Phenolamides, also known as phenylamides or hydroxycinnamic acid amides, are ubiquitous secondary metabolites in plants. All these phenolamide synthesis enzymes belong to the acyl-coenzyme A (CoA)-dependent BAHD acyltransferases family, which was named according to the first letter of each of its first four biochemically characterized enzymes: Benzylalcohol O-acetyltransferase, Anthocyanin O-HCT, HCT of anthranilate, and Deacetylvindoline 4-O-acetyltransferase. It has been established that BAHD acyltransferases catalyze the transfer of acyl groups from acyl-donors (Acyl-CoA) to various acyl-acceptors. In this study, we first performed structural analyses on two representative BAHD family enzymes, the Arabidopsis mono-/di-acyltransferase-SDT (AtSDT) and poly acyltransferase-SHT (AtSHT), then explored the acceptor-molecule specificity and potential molecular mechanisms of multisite acylation by structure-based mutagenesis approaches, and, finally, successfully predicted and varified the acyl acceptor substrates of two uncharacterized BAHD family transferases in Arabidopsis using our prediction methods on the basis of a sequence similarity network (SSN) and of structure modeling.

In contrast to the mono- or di- substituted phenolamides, which seem to be widely distributed in different organs, the poly-substituted phenolamides, tri-substituted spermidine, and tetra-substituted spermidine were found to be restricted to the flower pollen coat. Spermidine/spermine hydroxycinnamoyl transferases (SHT), accounting for the synthesis of tri- or tetra- substituted spermidine/spermidine, have been identified and studied in Arabidopsis thaliana (AtSHT), Malus domestica (MdSHT), and Cichorium intybus (CiSHT; Grienenberger et al., 2009; Elejalde-Palmett et al., 2015; Delporte et al., 2018). In addition, the multisite acylation mechanisms of BAHD-family acyltransferases also remain poorly understood until now.

> MAPITFRKSYTIVPAEPTWSGRFPLAEWDQVGTITHIPTLYFYDKPSESFQGNVVEILKTSLSRVLVHFYPMAGRLRWLPRGRFELNCNAEGVEFIEAESEGKLSDFKDFSPTPEFENLMPQVNYKNPIETIPLFLAQVTKFKCGGISLSVNVSHAIVDGQSALHLISEWGRLARGEPLETVPFLDRKILWAGEPLPPFVSPPKFDHKEFDQPPFLIGETDNVEERKKKTIVVMLPLSTSQLQKLRSKANGSKHSDPAKGFTRYETVTGHVWRCACKARGHSPEQPTALGICIDTRSRMEPPLPRGYFGNATLDVVAASTSGELISNELGFAASLISKAIKNVTNEYVMIGIEYLKNQKDLKKFQDLHALGSTEGPFYGNPNLGVVSWLTLPMYGLDFGWGKEFYTGPGTHDFDGDSLILPDQNEDGSVILATCLQVAHMEAFKKHFYEDI> NV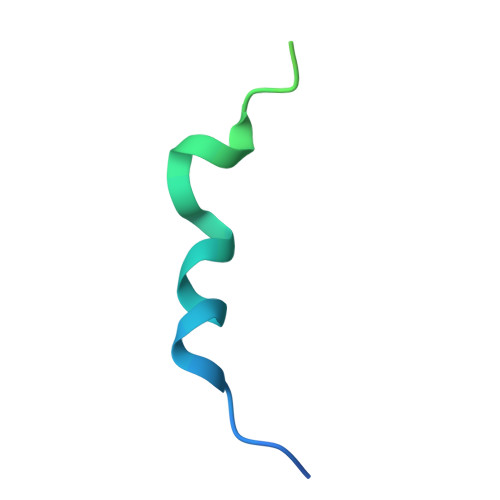QKYIPPTILTKRRNMESFNDCKVNTKDIISFKDVNQEYETWLDKHLSLAKDRD>[2x]GPMEADIITNLRCRLKEAEEERLKAAQYGLQLVESQNELQNQLDKCRNEMMTMTESYEQEKYTLQREVELKSRMLESLSCECEAIKQQQKMHLEKLEEQLSR

Here, we addressed the organization and regulation of Spindly, a farnesylated mitotic regulator of DD (605 residues in humans). In early mitosis, Spindly promotes recruitment of DD to kinetochores, the structures that connect chromosomes to spindle microtubules. This function of Spindly is enabled by the 800-kD hexameric ROD–Zwilch–ZW10 (RZZ) cargo complex, to which Spindly binds directly through its farnesylated C-terminal region. In conclusion, we have studied in mechanistic detail the basis of Spindly activation at the kinetochore and shown it to reflect a structural transition from a closed to an open conformation.

We then determined the crystal structure of human Spindly1–100 (only residues 2–97 were clearly resolved in the electron density), a fragment containing both the CC1 box and the HBS1. Spindly1–100 forms a parallel dimeric coiled-coil, similar in its outline to that observed in structures of other adaptors captured in complex with DD. Thus, both SpindlyFL and an N-terminal segment of Spindly are stable dimers. In Spindly, Ala23 and Gly27 in the CC1 box occupy a and d positions within the coiled-coil’s heptad repeats, similarly to Ala43 and Gly47 in BicD2, a pattern also conserved in BICDL1 and BICD1. This unusual composition for a and d residues generates a cavity along the BICD2 coiled-coil axis that interacts with aromatic and hydrophobic LIC side chains. Indeed, Spindly and BICD2 interact with the LIC with similar affinity. The ≈23 nm CC1a coiled-coil, partly captured in our crystal structure, is predicted to encompass the majority of the long axis of the Spindly dimer (≈28 nm), in good agreement with values derived from 2D class averages of negatively stained Spindly samples and small-angle x-ray scattering experiments for both SpindlyFL and Spindly1–440. Collectively, these observations indicate that the Spindly auto-inhibition mechanism involves a tight intramolecular interaction of the conserved Dynein-binding CC1 box with a regulatory segment of the Spindly CC2 coiled-coil roughly comprised between residues 276 and 306.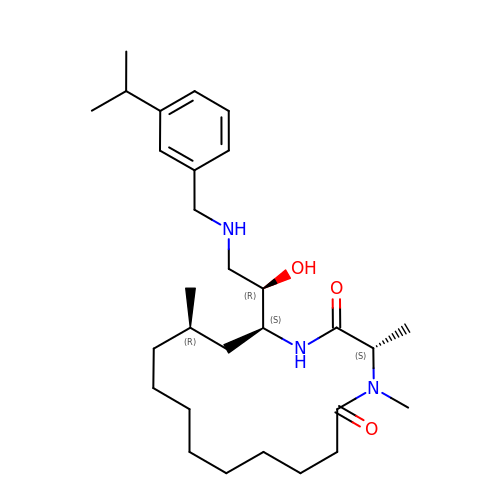(3S,14R,16S)-16-[(1R)-1-hydroxy-2-{[3-(1-methylethyl)benzyl]amino}ethyl]-3,4,14-trimethyl-1,4-diazacyclohexadecane-2,5-dione | C29 H49 N3 O3 | LHBBUGLYVFZUTH-GXVHRJHYSA-N> MAPWKIEEVKTLKGLIKSKPVVAIVDMMDVPAPQLQEIRDKIRDKVKLRMSRNTLIIRALKEAAEELNNPKLAELANYVERGAAILVTDMNPFKLYKLLEENKSPAPVRGGQIAPCDIKVEKGSTGMPPGPFLGELKSVGIPAAIE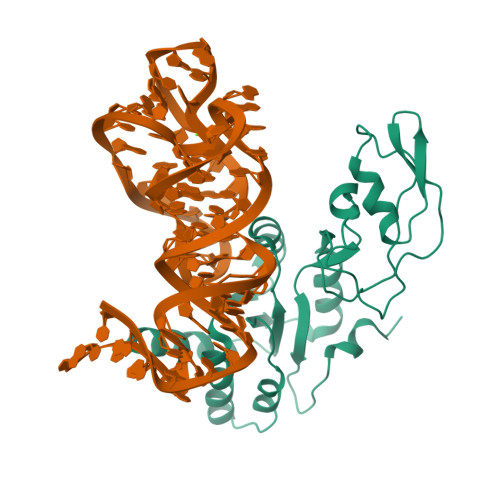KGKIAIKEDKVVVKKGEVVSPKLAAVLDRLGIKPIKVGLNILAVYEDGIIYTPDVLKVDEEKLLADI>[3x]MSHHHHHHSMQRTKIVVKVHMPCGKSRAKALALAASVNGVDSVEITGEDKDRLVVVGRGIDPVRLVALLREKCG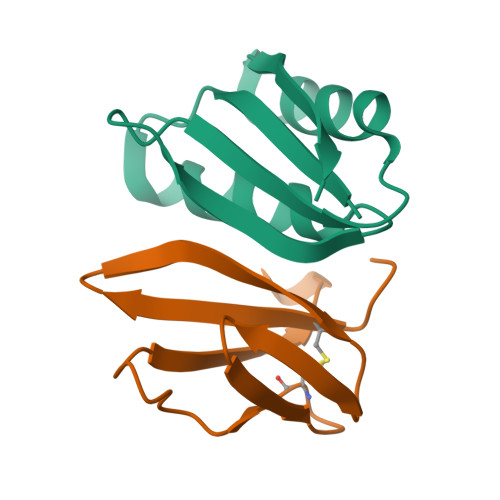LAELLMVELV;>[2x]MAWKDCIIQRYKDGDVNNIYTANRNEEITIEEYKVFVNEACHPYPVILPDRSVLSGDFTSAYLEHHHHHH>[3x]MSLDFWLYKQAQQNGHHIAITDGQESYTYQNLYCEASLLAKRLKAYQQSRVGLYIDNSIQSIILIHACWLANIEIAMINTRLTPNEMTNQMRSIDVQLIFCTLPLELRGFQIVSLDDIEFAGRDITTNGLLDNTMGIQYD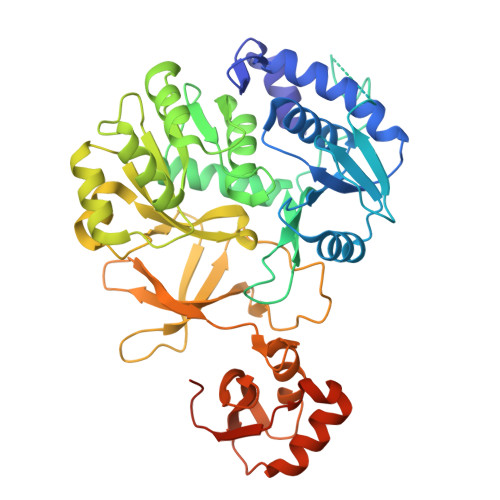TSNETVVPKESPSNILNTSFNLDDIASIMFTSGTTGPQKAVPQTFRNHYASAIGCKESLGFDRDTNWLSVLPIYHISGLSVLLRAVIEGFTVRIVDKFNAEQILTMIKNERITHISLVPQTLNWLMQQGLHEPYNLQKILLGGAKLSATMIETALQYNLPIYNSFGMTETCSQFLTATPEMLHARPDTVGMPSANVDVKIKNPNKEGHGELMIKGANVMNGYLYPTDLTGTFENGYFNTGDIAEIDHEGYVMIYDRRKDLIISGGENIYPYQIETVAKQFPGISDAVCVGHPDDTWGQVPKLYFVSESDISKAQLIAYLSKHLAKYKVPKHFEKVDTLPYTSTGKLQRNKLYREGHHHHHH> SFDCGKPQVEPKKCPGAVVGGCVAYPHSWPWQVSLRTRFGMHFCGGTLISPEWVLTAAHCLEKSPRPSSYKVILGAHQEVNLEPHVQEIEVSRLFLEPTRKDIALLKLSSPAVITDKVIPACLPSPNYVVADRTECFITGWGETQGTFGAGLLMEAQLPVIENKVCNRYEFLNGRVQSTELCAGHLAGGTDSCQGDSGGPLVCFEKDKYILQGVTSWGLG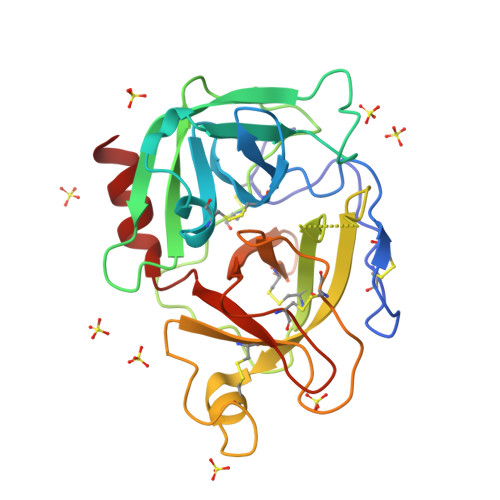CARPNKPGVYVRVSRFVTWIEGVMRNN>GSDEIDLSALRDPAGIFELVELVGNGTYGQVYKGRHVKTGQLAAIKVMDVTGDEEEEIKQEINMLKKYSHHRNIATYYGAFIKKNPPGMDDQLWLVMEFCGAGSVTDLIKNTKGNTLKEEWIAYICREILRGLSHLHQHKVIHRDIKGQNVLLTENAEVKLVDFGVSAQLDRTVGRRNTFIGTPYWMAPEVIACDENPDATYDFKSDLWSLGITAIEMAEGAPPLCDMHPMRALFLIPRNPAPRLKSKKWSKKFQSFIESCLVKNHSQRPATE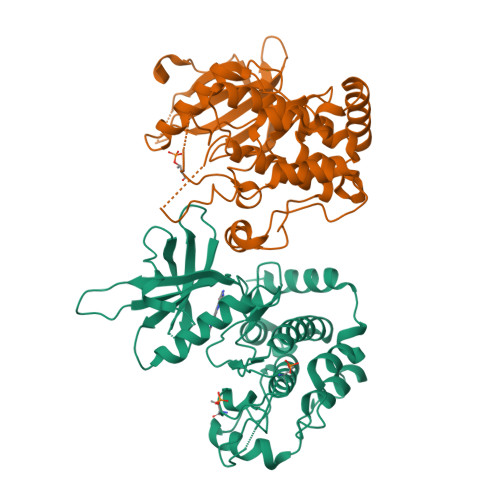QLMKHPFIRDQPNERQVRIQLKDHIDRTKKKRG[2x]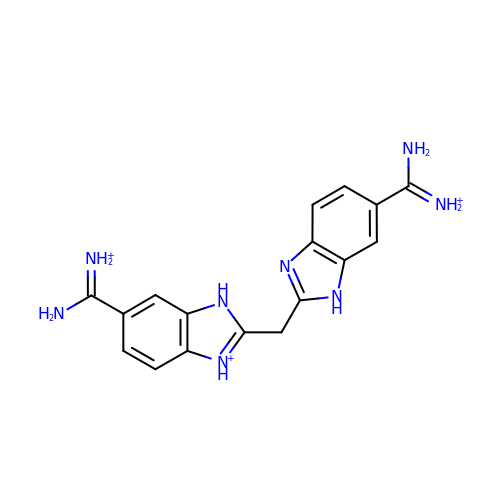BIS(5-AMIDINO-BENZIMIDAZOLYL)METHANE | C17 H19 N8 | QZKOOEFIMWKZPK-UHFFFAOYSA-Q>REWFLHRNSLIVLADVALFLALYHFLPFEHNVVLGISMLAFIAVLWLTEALHVTVTAILVPVMAVFFGIFETQAALNNFANSIIFLFLGGFALAAAMHHQGLDKVIADKVLAMAQGKMSVAVFMLFGVTALLSMWISNTATAAMMLPLVLGVLSKVDADKQRSTYVFVLLGVAYSASIGGIATLVGSPPNAIAAAEVGLSFTDWMKFGLPTAMMMLPMAIAILYFLLKPTLNGMFELDRAPVNWDKGKVVTLGIFGLTVFLWIFSSPINAALGGFKSFDTLVALGAILMLSFARVVHWKEIQKTADWGVLLLFGGGLCLSNVLKQTGTSVFLANALSDMVSHMGIFVVILVVATFVVFLTEFASNTASAALLIPVFATVAEAFGMSPVLLSVLIAVAASCAFMLPVATPPNAIVFASGHIKQSEMMRVGLYLNIACIGLLTAIAMLFWQ[4x]

The mammalian SLC13 proteins are members of the larger divalent-anion sodium symporter (DASS) family. DASS proteins typically have a molecular weight of 45–65 kDa and form obligate homodimers. Each protomer consists of a scaffold and a transport domain. Structural information, along with cross-linking and computer modeling, indicates that DASS proteins operate in an elevator-type transport mechanism (Reyes et al., 2009; Drew and Boudker, 2016; Garaeva and Slotboom, 2020).

Finally, to obtain clear density of substrate in the binding site of VcINDY, we crystallized the protein in complex with sodium and terephthalate, and solved the X-ray structure to 3.92 Å resolution by molecular replacement. With two carboxylate moieties at approximately the same distance as those of native substrates, we hypothesized the terephthalate would bind within the VcINDY binding site, while its large benzene ring would provide stronger electron density than succinate, fumarate, or malate. In the transport domain, the two carboxylate moieties of the bound substrate are coordinated by two conserved Ser-Asn-Thr (SNT) motifs, which also form part of the Na+-binding sites Na1 and Na2.methyl 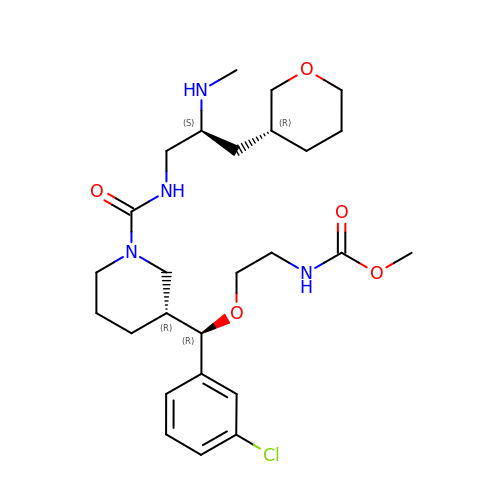(2-{(R)-(3-chlorophenyl)[(3R)-1-({(2S)-2-(methylamino)-3-[(3R)-tetrahydro-2H-pyran-3-yl]propyl}carbamoyl)piperidin-3-yl]methoxy}ethyl)carbamate | C26 H41 Cl N4 O5 | NXWASIVXQMMPLM-ZXMXYHOLSA-N> GATAGAVSARAAEQQRLQRIVDAVARQEPRISWAAGLRDDGTTTLLVTDLAGGWIPPHVRLPANVTLLEPTARRRDADVIDLLGAVVAVAAHESNT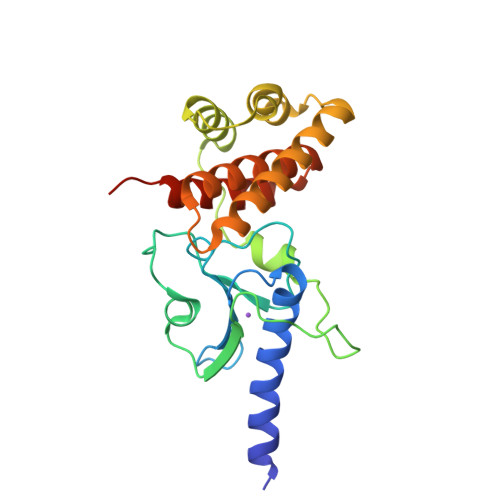YVAEPGPDAPALTGDRSARSAIPKVDEFGPTLVEAVRRRDSLPRIAQAIALPAVRKTGVLENEAELLHGCITAVKESVLKAYPSHELTAVGDWMLLAAIEALIDEQDYLANYHLAWYAVTTRRGGSRGFAA> SMKQTGYLTIGGQRYQAEINDLENLGEMGSGTCGQVWKMRFRKTGHVIAVKQMRRSGNKEENKRILMDLDVVLKSHDCPYIVQCFGTFITNTDVFIAMELMGTCAEKLKKRMQGPIPERILGKMTVAIVKALYYLKEKHGVIHRDVKPSNILLDERGQIKLCDFGISGRLVDSKAKTRSAGCAAYMAPERIDPPDPTKPDYDIRADVWSLGISLVELATGQFPYKNCKTDFEVLTKVLQEEPPLLPGHMGFSGDFQSFVKDCLTKDHRKRP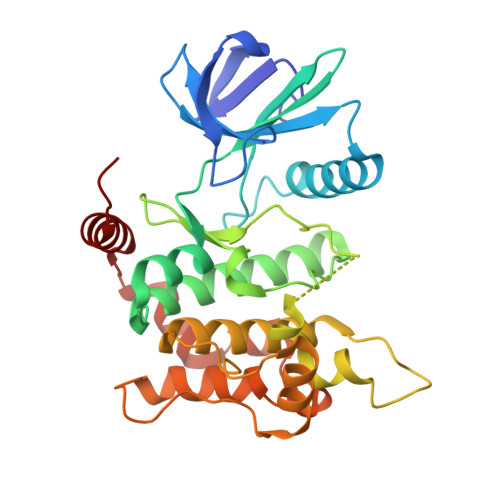KYNKLLEHSFIKRYETLEVDVASWFKDVMAKTESPR> MSRSKRDNNFYSVEIGDSTFTVLKRYQNLKPIGSGAQGIVCAAYDAILERNVAIKKLSRPFQNQTHAKRAYRELVLMKVVNHKNIIGLLNVFTPQKSLEEFQDVYIVMELMDANLSQVIQMELDHERMSYLLYQMLVGIKHLHSAGIIHRDLKPSNIVVKSDATLKILDFGLARTAGTSFMMTPYVVTRYYRAPEVILGMGYKENVDIWSVGCIMGEMIKGGVLFPGTDHIDQWNKVIEQLGTPSPEFMKKLQPTVRTYVENRPKYAGYSFEKLFPDVLFPADSEHNKLKASQARDLLSKMLVIDASKRISVDEAL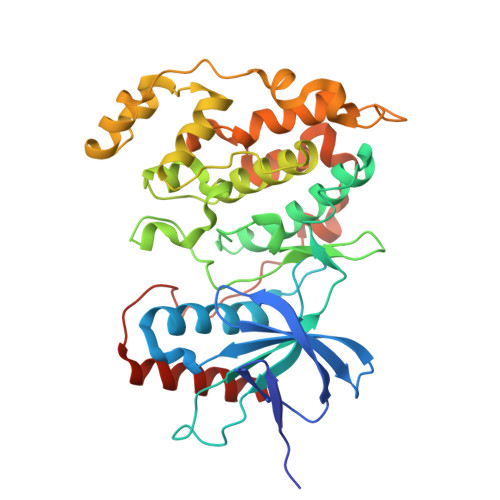QHPYINVWYDPSEAEAPPPKIPDKQLDEREHTIEEWKELIYKEVMDLEHHHHHH>MSGIDPKRFGKVAVLLGGDSAEREVSLNSGRLVLQGLRDAGIDAHPFDPAQRPLAALKDEGFVRAFNALHGGYGENGQIQGALDFYGIRYTGSGVLGSALGLDKFRTKLVWQQTGIPTPPFETVMRGDDYAARAQDIVAKLGVPLFVKPASEGSSVAVEKVKSADALPAALEEAAKHDKIVIVEKSIEGGGEYTACIAADLDLPLIRIVPAGEFYDYHAKYIANDTQYLIPCGLDAAKEAEFKRIARRAFDVLGCTDWGRADFMLDAAGNPYFLEVNTAPGMTDHSLPPKAARAVGIGYSELVVKVLSLTLD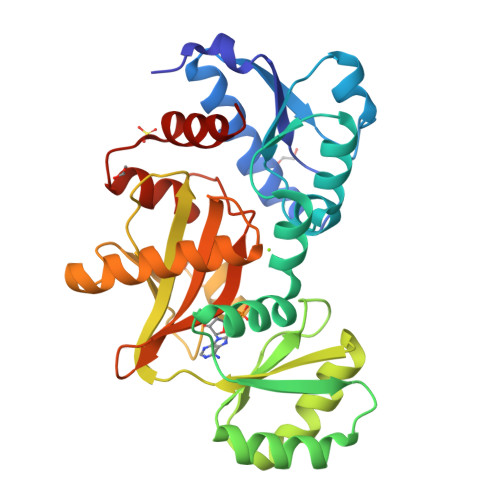[2x]3-[(R)-[(2E,4S)-2-imino-4-methyl-6-oxo-4-(propan-2-yl)-1,3-diazinan-1-yl](phenyl)methyl]-N-[(1S)-1-phenylethyl]benzamide 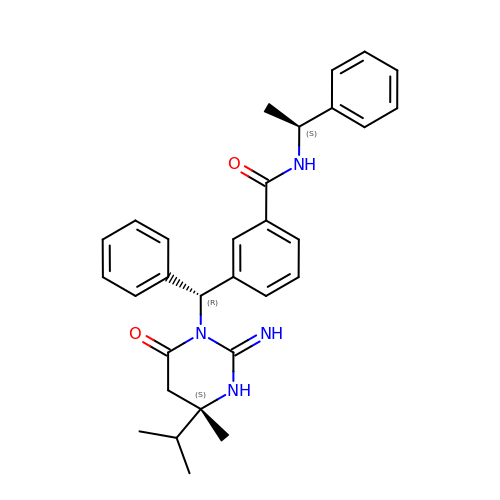| C30 H34 N4 O2 | GYWZRASVOLJLOW-HAALKUMUSA-N> MPRPRVLLLGDPARHLDDLWSDFQQKFEVIPANLTTHDGFKQALREKRYGDFEAIIKLAVENGTESYPWNADIISHLPSSLKVFAAAGAGFDWLDLDALNERGVAFANSRGAGDTATSDLALYLILSVFRLASYSERAARTGDPETFNRVHLEIGKSAHNPRGHVLGAVGLGAIQKEIARKAVHGLGMKLVYYDVAPADA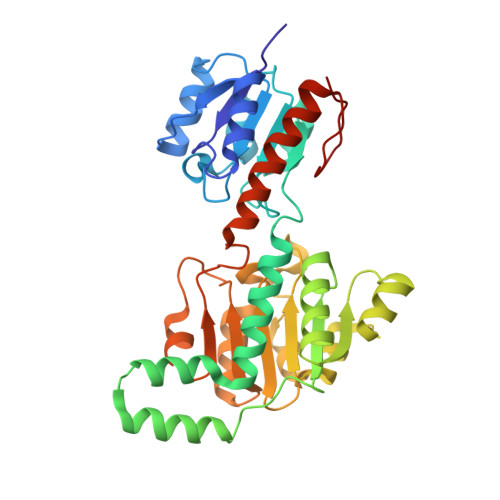ETEKALGAERVDSLEELARRSDCVSVSVPYMKLTHHLIDEAFFAAMKPGSRIVNTARGPVISQDALIAALKSGKLLSAGLDVHEFEPQVSKELIEMKHVTLTTHIGGVAIETFHEFERLTMTNIDRFLLQGKPLLTPAGKVFAPSSAA> MHHHHHHHHGDYKDDDDKGTDEEEDGAGAEESGQPRSFMRLNDLSGAGGRPGPGSAEKDPGSADSEAEGLPYPALAPVVFFYLSQDSRPRSWCLRTVCNPWFERISMLVILLNCVTLGMFRPCEDIACDSQRCRILQAFDDFIFAFFAVEMVVKMVALGIFGKKCYLGDTWNRLDFFIVIAGMLEYSLDLQNVSFSAVRTVRVLRPLRAINRVPSMRILVTLLLDTLPMLGNVLLLCFFVFFIFGIVGVQLWAGLLRNRCFLPENFSLPLSVDLERYYQTENEDESPFICSQPRENGMRSCRSVPTLRGDGGGGPPCGLDYEAYNSSSNTTCVNWNQYYTNCSAGEHNPFKGAINFDNIGYAWIAIFQVITLEGWVDIMYFVMDAHSFYNFIYFILLIIVGSFFMINLCLVVIATQFSETKQRESQLMREQRVRFLSNASTLASFSEPGSCYEELLKYLVYILRKAARRLAQVSRAAGVRVGLLSSPAPLGGQETQPSSSCSRSHRRLSVHHLVHHHHHHHHHYHLGACQSSCKISSPCLKADSGACGPDSCPYCARAGAGEVELADREMPDSDSEAVYEFTQDAQHSDLRDPHSRRQRSLGPDAEPSSVLAFWRLICDTFRKIVDSKYFGRGIMIAILVNTLSMGIEYHEQPEELTNALEISNIVFTSLFALEMLLKLLVYGPFGYIKNPYNIFDGVIVVISVWEIVGQQGGGLSVLRTFRLMRVLKLVRFLPALQRQLVVLMKTMDNVATFCMLLMLFIFIFSILGMHLFGCKFASERDGDTLPDRKNFDSLLWAIVTVFQILTQEDWNKVLYNGMASTSSWAALYFIALMTFGNYVLFNLLVAILVEGFQAEGDANKSESEPDFFSPSLDGDGDRKKCLALVSLGEHPELRKSLLPPLIIHTAATPMSLPKSTSTGLGEALGPASRRTSSSGSAEPGAAHEMKSPPSARSSPHSPWSAASSWTSRRSSRNSLGRAPSLKRRSPSGERRSLLSGEGQESQDEEESSEEERASPAGSDHRHRGSLEREAKSSFDLPDTLQVPGLHRTASGRGSASEHQDCNGKSASGRLARALRPDDPPLDGDDADDEGNLSKGERVRAWIRARLPACCLERDSWSAYIFPPQSRFRLLCHRIITHKMFDHVVLVIIFLNCITIAMERPKIDPHSAERIFLTLSNYIFTAVFLAEMTVKVVALGWCFGEQAYLRSSWNVLDGLLVLISVIDILVSMVSDSGTKILGMLRVLRL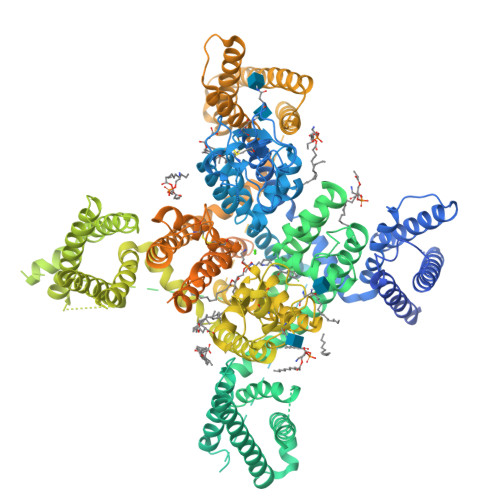LRTLRPLRVISRAQGLKLVVETLMSSLKPIGNIVVICCAFFIIFGILGVQLFKGKFFVCQGEDTRNITNKSDCAEASYRWVRHKYNFDNLGQALMSLFVLASKDGWVDIMYDGLDAVGVDQQPIMNHNPWMLLYFISFLLIVAFFVLNMFVGVVVENFHKCRQHQEEEEARRREEKRLRRLEKKRRNLMLDDVIASGSSASAASEAQCKPYYSDYSRFRLLVHHLCTSHYLDLFITGVIGLNVVTMAMEHYQQPQILDEALKICNYIFTVIFVLESVFKLVAFGFRRFFQDRWNQLDLAIVLLSIMGITLEEIEVNASLPINPTIIRIMRVLRIARVLKLLKMAVGMRALLDTVMQALPQVGNLGLLFMLLFFIFAALGVELFGDLECDETHPCEGLGRHATFRNFGMAFLTLFRVSTGDNWNGIMKDTLRDCDQESTCYNTVISPIYFVSFVLTAQFVLVNVVIAVLMKHLEESNKEAKEEAELEAELELEMKTLSPQPHSPLGSPFLWPGVEGPDSPDSPKPGALHPAAHARSASHFSLEHPTMQPHPTELPGPDLLTVRKSGVSRTHSLPNDSYMCRHGSTAEGPLGHRGWGLPKAQSGSVLSVHSQPADTSYILQLPKDAPHLLQPHSAPTWGTIPKLPPPGRSPLAQRPLRRQAAIRTDSLDVQGLGSREDLLAEVSGPSPPLARAYSFWGQSSTQAQQHSRSHSKISKHMTPPAPCPGPEPNWGKGPPETRSSLELDTELSWISGDLLPPGGQEEPPSPRDLKKCYSVEAQSCQRRPTSWLDEQRRHSIAVSCLDSGSQPHLGTDPSNLGGQPLGGPGSRPKKKLSPPSITIDPPESQGPRTPPSPGICLRRRAPSSDSKDPLASGPPDSMAASPSPKKDVLSLSGLSSDPADLDP> GGCCGAC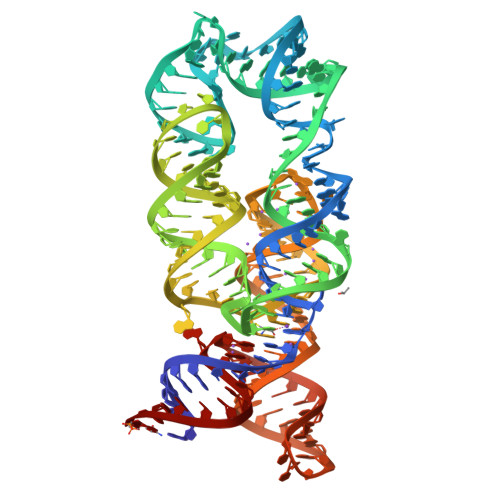GGAGGCGCGCCCGAGAUGAGUAGGCUGUCCCAUCAGGGGAGGAAUCGGGGACGGCUGAAAGGCGAGGGCGCCGAAGGGUGCAGAGUUCCUCCCGCUCUGCAUGCCUGGGGGUAUGGGGAAUACCCAUACCACUGUCACGGAGGUCUCUCCGUGGAGAGCCGUCGGUC> VEVTSRLTVAGSDAKCDFFTPATQD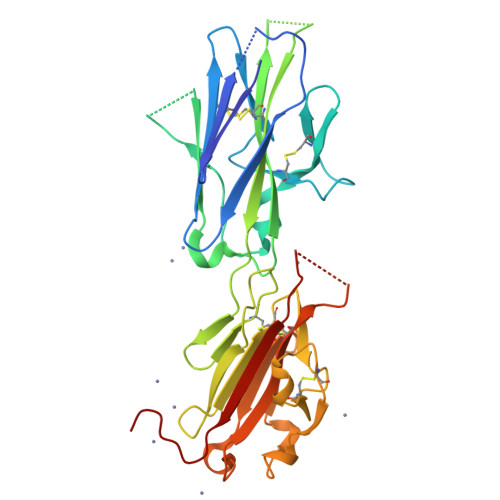SPPVSGSLTLSKGRMTATFECSATQALSISTIPTNIEQNVCDPKKTTNGTVCQFGANGSAGTEVTLKDLLETDRIVNWKVNEQREESNKSQKWSLELHNEDLPLTDKAFVVGCQATSAARGTESGKTAACKLTVNVEARASSLAENNVVTCAYGKGSNPNPVEVEMSTEKNTLTINCGSDGSLQPTTYAEEYCVADSKDVNRCSTTRFVEIFPKFLKSWWVTETQKRTSATLTIPQTDLPEADQQFLVGCVPKKTAPEDPKKDKESGTETAAPTSCTVLVTVKAHHHHHH> MALPLLNYAPKSQNVRVEGYEIGSEEKPVVFTTENILSSSDMDNLIEAA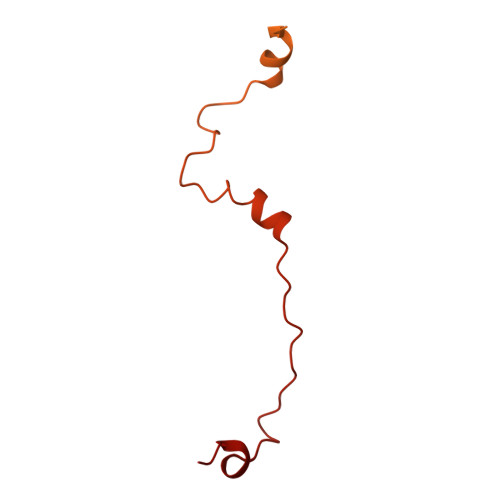YRQIFFHAFKWDREKVLESQLRNGQITVRDFVRGLLLSNTFRNSFYEKNSNYRFVEHCVQKILGRDVYSEREKIAWSIVVATKGYQGLIDDLLNSDEYLNNFGYDTVPYQRRRNLPGREAGELPFNIKSPRYDAYHRRQLGFPQIVWQNEVRRFIPQEKKLTAGNPMNFLGMARSINPAANTIPKVSAQNINIEASVPRR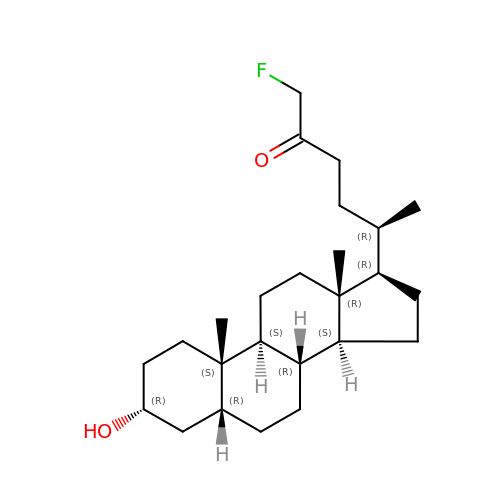(5R)-1-fluoro-5-[(1R,3aS,3bR,5aR,7R,9aS,9bS,11aR)-7-hydroxy-9a,11a-dimethylhexadecahydro-1H-cyclopenta[a]phenanthren-1-yl]hexan-2-one (non-preferred name) | C25 H41 F O2 | YECICDGDDQGLJC-QIAJLKNUSA-N2-{[(5Z,8Z,11Z,14Z)-icosa-5,8,11,14-tetraen-1-yl]oxy}propane-1,3-diol 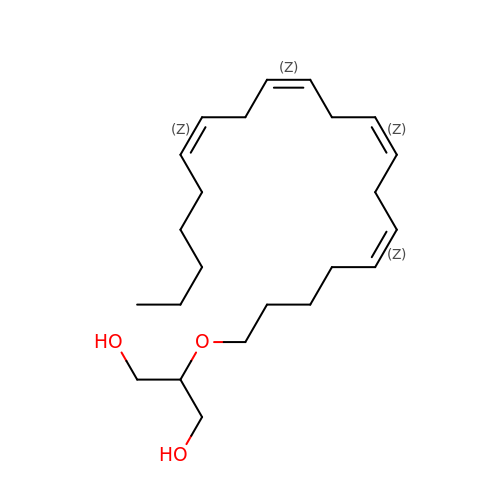| C23 H40 O3 | CUJUUWXZAQHCNC-DOFZRALJSA-N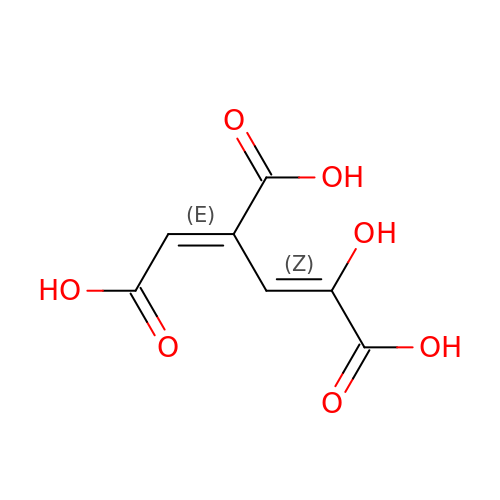(1E,3Z)-4-hydroxybuta-1,3-diene-1,2,4-tricarboxylic acid | C7 H6 O7 | QWLUKZXOQAQUFQ-NAOWAUKJSA-N> MQISSDYIPDSKFYKVEAIVRPWRIQQVSSALLKIGIRGVTVSDVRGFGAQGGSTERHGGSEFSEDKFVAKVKMEIVVKKDQVESVINTIIEGARTGEIGDGKIFVLPVSDVIRVRTGER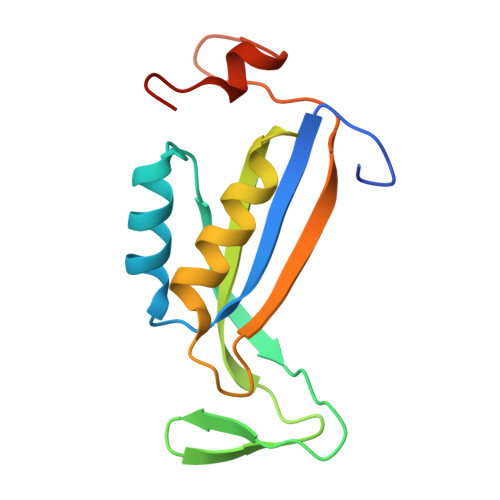GEKAEKMTGDMLSPS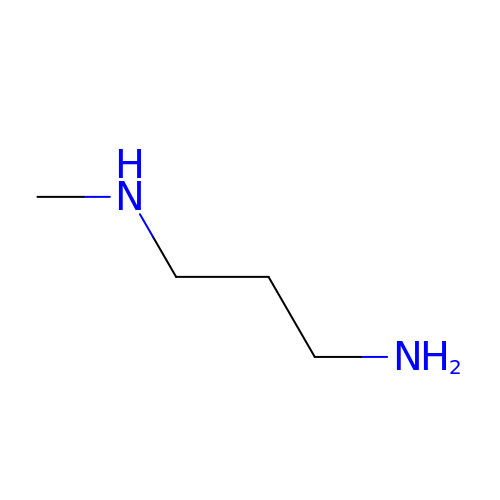N-methylpropane-1,3-diamine | C4 H12 N2 | QHJABUZHRJTCAR-UHFFFAOYSA-N>[6x]MDHAPERFDATPPAGEPDRPALGVLELTSIAR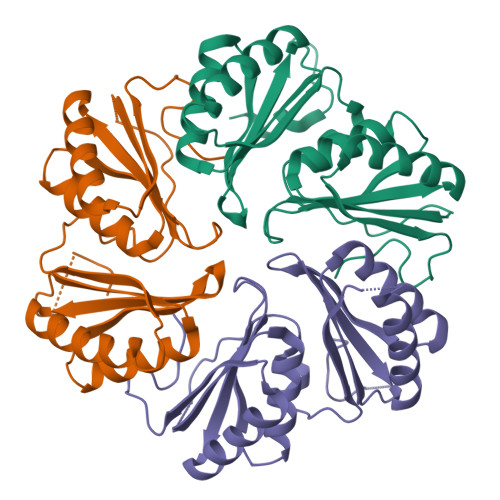GITVADAALKRAPSLLLMSRPVSSGKHLLMMRGQVAEVEESMIAAREIAGAGSGALLDELELPYAHEQLWRFLDAPVVADAWEEDTESVIIVETATVCAAIDSADAALKTAPVVLRDMRLAIGIAGKAFFTLTGELADVEAAAEVVRERCGARLLELACIARPVDELRGRLFF> DWATLSLEKLLKEKQALKSQISEKQRHCLELQISIV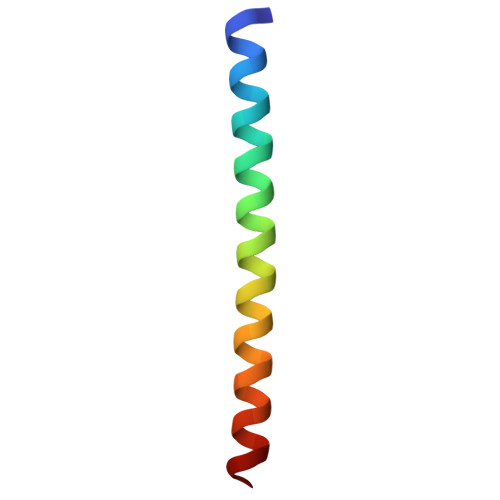ELEK>GPGADRAQDHNNNNTPRNSNY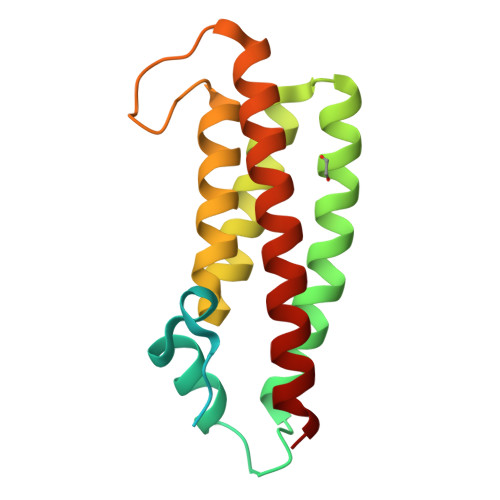VVEEEEVSEEEEEAIMMPDFGDHVDTSIFGQILEMDEGDDHDFSAPLVLNFFEQAEETFQKMETALNNKDLPELSKLGHFLKGSSATLGFTKIRDSCQLIQQYGHGLNVDGSSEPDEGVCLKKIAEALASARVDTVALHKMMREFFEY[4x]R-ETHYL N,N-DIMETHYLPHOSPHONAMIDATE | C4 H12 N O2 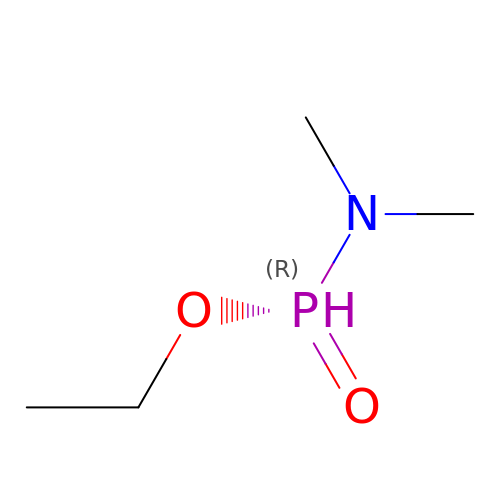P | VJBIKDDUGQICEU-UHFFFAOYSA-N> SGQPICGNGMVEQGEECDCGYSDQCKDECCYDANQPEGKKCKLKPGKQCSPSQGPCCTAHCAFKSKTEKCRDDSDCAKEGICNGITALCPASDPKPNFTDCNRHTQVCINGQCAGSICEKHGLEECTCASSDGKDDKELCHVCCMKKMEPSTCASTGSVQWNKYFLGRTITLQPGSPCND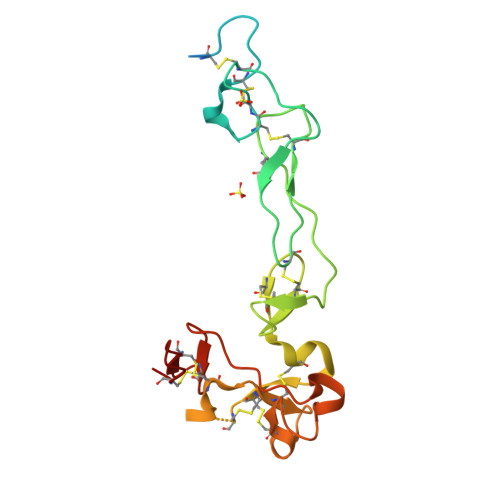FRGYCDVFMRCR> GSMPLLLDDGDPKAQTGFDLSTATTLFWRPVPVHVKQQDREDVLEELTFRILTGVAKQNHNLRILRIHISSDSDLFFLHTLEV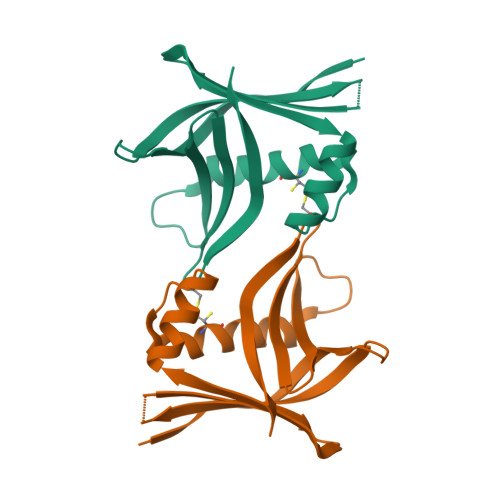SEEDFQSLKNDQGILVDFASFPGCIISLLEKCILAQPGDSPRFQAVLTIRGGESVFKIVEINDCKQLPHITLAFRPGN>MNKLVGLLVSSLFLASILIGIAPAITTTALTPPVSAGGIQAYLLTGSGAPASGLVLFVVNVSNIQVSSSNVTNVISTVVSNIQINAKTENAQTGATTGSVTVRFPTSGYNAYYDSVDKVVFVVVSFLYPYTTTSVNIPLSYLSKYLPGLLTAQPYDETGAQVTSVSSTPFGSLIDTSTGQQILGTNPVLTSYNSYTTQANTNMQEGVVSGTLTSFTLGGQSFSGSTVPVILYAPFIFSNSPYQAGLYNPMQVNGNLGSLSSEAYYHPVIWGRALINTTLIDTYASGSVPFTFQLNYSVPGPLTINMAQLAWIASINNLPTSFTYLSYKFSNGYESFLGIISNSTQLTAGALTINPSGNFTINGKKFYVYLLVVGSTNSTTPVEYVTKLVVEYPSSTNFLPQGVTVTTSSNKYTLPVYEIGGPAGTTITLTGNWYSTPYTVQITVGSTPTLTNYVSQILLKAVAYEGINVSTTQSPYYSTAILSTPPSEISITGSSTITAQGKLTATSASATVNLLTNATLTYENIPLTQYSFNGIIVTPGYAAINGTTAMAYVIGALYNKTSDYVLSFAGSQEPMQVMNNNLTEVTTLAPFGLTLLAPSVPATETGTSPLQLEFFTVPSTSYIALVDFGLWGNLTSVTVSAYDTVNNKLSVNLGYFYGIVIPPSISTAPYNYQNFICPNNYVTVTIYDPDAVLDPYPSGSFTTSSLPLKYGNMNITGAVIFPGSSVYNPSGVFGYSNFNKGAAVTTFTYTAQSGPFSPVALTGNTNYLSQYADNNPTDNYYFIQTVNGMPVLMGGLSIVASPVSASLPSSTSSPGFMYLLPSAAQVPSPLPGMATPNYNLNIYITYKIDGATVGNNMINGLYVASQNTLIYVVPNGSFVGSNIKLTYTTTDYAVLHYFYSTGQYKVFKTVSVPNVTANLYFPSSTTPLYQLSVPLYLSEPYYGSPLPTYIGLGTNGTSLWNSPNYVLFGVSAVQQYLGFIKSISVTLSNGTTVVIPLTTSNMQTLFPQLVGQELQACNGTFQFGISITGLEKLLNLNVQQLNNSILSVTYHDYVTGETLTATTKLVALSTLSLVAKGAGVVEFLLTAYPYTGNITFAPPWFIAENVVKQPFMTYSDLQFAKTNPSAILSLSTVNITVVGLGGKASVYYNSTSGQTVITNIYGQTVATLSGNVLPTLTELAAGNGTFTGSLQFTIVPNNTVVQIPSSLTKTSFAVYTNGSLAIVLNGKAYSLGPAGLFLLPFVTYTGSAIGANATAIITVSDGVGTSTTQVPITAENFTPIRLAPFQVPAQVPLPNAPKLKYEYNGSIVITPQQQVLKIYVTSILPYPQEFQIQAFVYEASQFNVHTGSPTAAPVYFSYSAVRAYPALGIGTSVPNLLVYVQLQGISNLPAGKYVIVLSAVPFAGGPVLSEYPAQLIFTNVTLTQ[4x];>MNKNLAILTPIVLLSLVLAPIAISAVTINGITFYSPVPNQTYKYGQQLVLSIQSQPNALVTLYVYDPKGNVVYNNVYQTNSSGGLTATIATFGSTPGFTTVGTYTVSLSVQGTTSESASVNVQYVPLTSTITATVVNQEGSPLAGATVQLYNTTSGSNTLVATQTTNSQGVATFTVLSFPGVTQTFKLVASLQGYAASTASVSITGQQNASVTITLVPAVVTIAPMYVIQNGTVIGSGPSLSSIVVYQGLPAYILAQVSFAGQRVTTAPVSAQVYYPNGTQTVKASVITSGKYAGMYNITIMPPTESVQNYVFQLLIVANYTTSSGQTLSTKYLMSVQANQNLQALVNKEISSLVQNITNLEKTVNNLQTQISTLNSSLSSLSQRITSLQNTLASLNSTISSLSGTASSLSSQLNALQGKISSLNSSITNLSGQLNSLQSKVNSLTPLVYGGIIAGIIGLIVAIVAIVLVYRKIS[3x]

Surface layers (S-layers) are resilient two-dimensional protein lattices that encapsulate many bacteria and most archaea. In archaea, S-layers usually form the only structural component of the cell wall and thus act as the final frontier between the cell and its environment. Sulfolobus acidocaldarius is a hyperthermophilic and acidophilic Crenarchaeon and thrives in acidic thermal soils and hot springs worldwide. The Sulfolobales S-layer lattice stands out from others because it is a two-component lattice, consisting of the S-layer-forming SlaA and the membrane anchor SlaB.

By combining SPA and STA with structural predictions, we built a complete S. acidocaldarius S-layer model. To get a handle on the structure of the entire S-layer, we used Alphafold v2.2.0 and SymmDock and predicted the monomeric and trimeric SlaB structure. The Alphafold predictions of the SlaB trimer superimposed remarkably well into the corresponding densities visible in our STA map at low threshold values, and flexible fitting using Namdinator further improved the fit. In the assembled lattice, SlaB trimers occupy alternating triangular pores around each hexagonal pore. The SlaB trimer has a tripod-like structure, with its long axis perpendicular to the planes formed by the membrane and SlaA. Three Ig-like domains branch away from the trimer’s symmetry axis and face the SlaA canopy, whereas three α-helices form a coiled coil, which at the predicted transmembrane region insert into the resolved exosome membrane. The lattice is a ~35-nm-thick macromolecular assembly, in which each SlaB trimer interacts with three SlaA dimers. This interaction may be mediated by the positively charged D6 dimerising domains of SlaA and the negatively charged N-terminal Ig-like D3 domains of SlaB. The new data confirm the overall p3 S-layer lattice symmetry, in which the unit cell contains one SlaB trimer and three SlaA dimers (SlaB3/3SlaA2). Because each SlaB monomer interacts with the dimerisation domains of SlaA dimers, the SlaB trimer occupancy of all triangular pores would likely be unfavourable due to steric hindrance.> MALSELALVRWLQESRRSRKLILFIVFLALLLDNMLLTVVVPIIPSYLYSIKHEKNATEIQTARPVHTA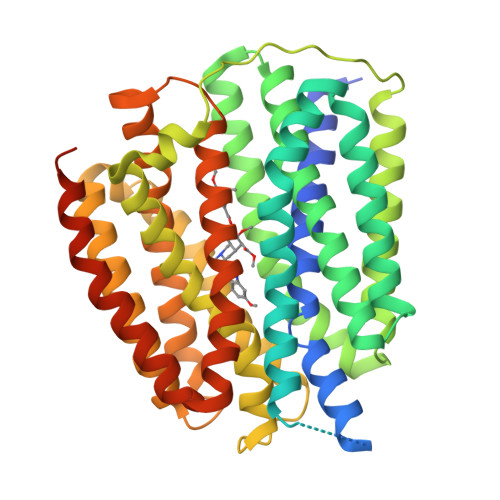SISDSFQSIFSYYDNSTMVTGNATRDLTLHQTATQHMVTNASAVPSDCPSEDKDLLNENVQVGLLFASKATVQLITNPFIGLLTNRIGYPIPIFAGFCIMFVSTIMFAFSSSYAFLLIARSLQGIGSSCSSVAGMGMLASVYTDDEERGNVMGIALGGLAMGVLVGPPFGSVLYEFVGKTAPFLVLAALVLLDGAIQLFVLQPSRVQPESQKGTPLTTLLKDPYILIAAGSICFANMGIAMLEPALPIWMMETMCSRKWQLGVAFLPASISYLIGTNIFGILAHKMGRWLCALLGMIIVGVSILCIPFAKNIYGLIAPNFGVGFAIGMVDSSMMPIMGYLVDLRHVSVYGSVCAIADVAFCMGYAIGPSAGGAIAKAIGFPWLMTIIGIIDILFAPLCFFLRSPPSRLEEELRRRTEGGSSDLEVLFQ>MSLYEWLNALPKAELHLHLEGTLEPELLFALAERNRIALPWNDVETLRKAYAFNNLQEFLDLYYAGADVLR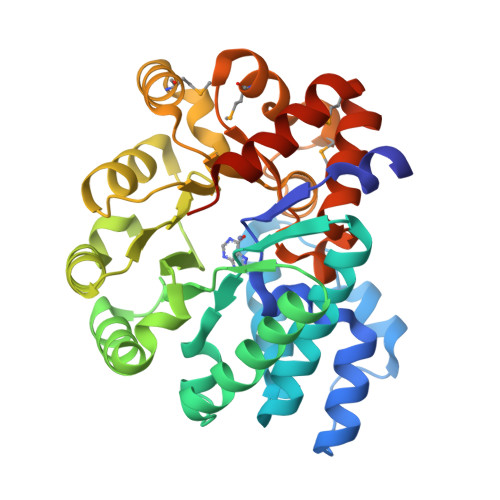TEQDFYDLTWAYLQKCKAQNVVHVEPFFDPQTHTDRGIPFEVVLAGIRAALRDGEKLLGIRHGLILSFLRHLSEEQAQKTLDQALPFRDAFIAVGLDSSEVGHPPSKFQRVFDRARSEGFLTVAHAGEEGPPEYIWEALDLLKVERIDHGVRAFEDERLMRRLIDEQIPLTVCPLSNTKLCVFDDMSQHTILDMLERGVKVTVNSDDPAYFGGYVTENFHALQQSLGMTEEQARRLAQNSLDARLVKEGHHHHHH[2x]> MTERTLKVLSPLHIGTGNELTPVDIYPRENIIHVLDTERLVNDLMNLGVELNEILALLKNPPGDAYIWKGYIEEFHLDPSDYSIYTLKIHGKIGRKSMQIKEFIKLNGRPYIPGSSLKGAIRTAVLYKALKECGDARAVMRVVSKVNGDVARDIGRSEDVLDYYMSFLSRARIDRKRADDLLEAIVFGMEPDRRSKIRYEPKRDPMKALIVRDSKPVGRKHLAVYHVEVIGNPQPIPIWVEAIEPGAA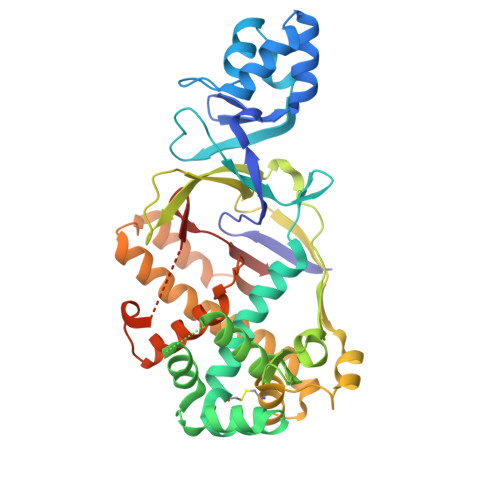TDVEIHVDTEALRLNADYFNGLLWECLKERGEPGEVFEDFLWEAVDEFYTAVMKYETIEVQKFGRYTSQVRSFYASLEDHSGHVLRLGWGSGWLAMTIGLLLVEKGYKWENVRKKLGLGKKPGGSGFSREFPKTRRLADGMPMGWVVLE>[2x]QPVVKSLLDSKGIHYNQGNPYNLLTPVIEKVKPGEQSFVGQHAATGCVATATAQIMKYHNYPNKGLKDYTYTLSSNNPYFNHPKNLFAAISTRQYNWNNILPTYSGRESNVQKMAISELMADVGISVDMDYGPSSGSAGSSRVQRALKENFGYNQSVHQINRSDFSKQDWEAQIDKELSQNQPVYYQGVGK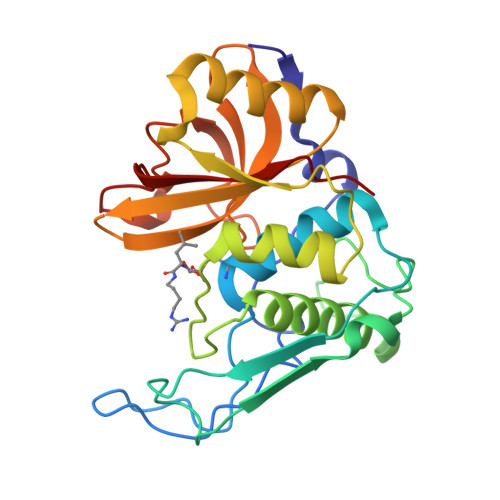VGGHAFVIDGADGRNFYHVNWGWGGVSDGFFRLDALNPSALGTGGGAGGFNGYQSAVVGIKP Using a phylogenomics-based approach and complementary structural techniques, we identify a family of dimeric hemoproteins comprising a domain of unknown function DUF2470. The heme iron is axially coordinated by two zinc-bound histidine residues, forming a distinct two-fold symmetric zinc-histidine-iron-histidine-zinc site. Together with structure-guided in vitro and in vivo experiments, we further demonstrate the existence of a functional link between heme binding by Dri1 (Domain related to iron 1, formerly ssr1698) and post-translational regulation of succinate dehydrogenase in the cyanobacterium Synechocystis, suggesting an iron-dependent regulatory link between photosynthesis and respiration. Given the ubiquity of proteins containing homologous domains and connections to heme metabolism across eukaryotes and prokaryotes, we propose that DRI (Domain Related to Iron; formerly DUF2470) functions at the molecular level as a heme-dependent regulatory domain. We heterologously expressed and purified the recombinant protein encoded by the Synechocystis gene dri1 (formerly known as ssr1698) and tested the heme-binding ability of this small, soluble protein (96 amino acids, 10 kDa).

The native structure devoid of heme is a single monomeric chain with a fold comparable to other DUF2470 structures in fusion proteins and comprises of three histidine residues (His16, His21, and His79; one on each alpha helix) that form a tetrahedral coordination site for a zinc ion. Looking at the sequence conservation of these residues, we observe strict conservation of His16 and His21 (numeration based on the Synechocystis protein sequence) throughout different phyla, with the exception of GBP. Radius of gyration (Rg) values from Guinier analyses and molecular weight estimations confirm that Dri1 without heme remains monomeric and heme-bound Dri1 is dimeric. Dimensionless Kratky plots further indicate that binding to heme decreases protein flexibility. We used homology modeling and docking analyses to predict candidate residues for a heme-free Dri1-SdhB1 heterodimer. SdhB1 residues, namely Cys214, Tyr215, and Glu219, were computationally predicted to interact with Dri1 zinc-binding residues (His16, His21, His79, and Glu76). However, mutations of the metal-binding site residues (His16Ala, His21Ala, or Glu76Ala) led to loss of an interaction, suggesting their involvement in complex formation. Therefore, under low cellular heme availability, Dri1 binds to SdhB, preventing SdhB docking to the membrane-bound domain HdrB.

>[4x]MADPLTPAISDRICKHMNEDHASAIALYAQVFGQQTDVTMAQMQAIDPTGMDLVVESEGGSKTIRIEFEQPLKDSEDAHQVLIAMAKQARSVGKNSAENLYFQ> TPATQPLINAE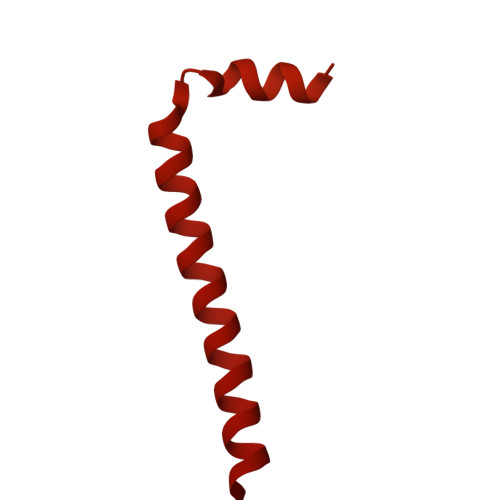PAVAAQTEQNPQVGQVMPGVQGADAPVVAQNGPSRDVKLTFAQIAPPPGSMVLRGINPNGSIEFGMRSDEVVTKAMLNLEYTPSPSLLPVQSQLKVYLNDELMGVLPVTKEQLGKKTLAQMPINPLFITDFNRVRLEFVGHYQDVCENPASTTLWLDVGRSSGLDLTYQTLNVKNDLSHFPVPFFDPRDNRTNTLPMVFAGAPDVGLQQASAIVASWFGSRSGWRGQNFPVLYNQLPDRNAIVFATNDKRPDFLRDHPAVKAPVIEMINHPQNPYVKLLVVFGRDDKDLLQAAKGIAQGNILFRGESVVVNEVKPLLPRKPYDAPNWVRTDRPVTFGELKTYEEQLQSSGLEPAAINVSLNLPPDLYLMRSTGIDMDINYRYTMPPVKDSSRMDISLNNQFLQSFNLSSKQEANRLLLRIPVLQGLLDGKTDVSIPALKLGATNQLRFDFEYMNPMPGGSVDNCITFQPVQNHVVIGDDSTIDFSKYYHFIPMPDLRAFANAGFPFSRMADLSQTITVMPKAPNEAQMETLLNTVGFIGAQTGFPAINLTVTDDGSTIQGKDADIMIIGGIPDKLKDDKQIDLLVQATESWVKTPMRQTPFPGIVPDESDRAAETRSTLTSSGAMAAVIGFQSPYNDQRSVIALLADSPRGYEMLNDAVNDSGKRATMFGSVAVIRESGINSLRVGDVYYVGHLPWFERLWYALANHPILLAVLAAISVILLAWVLWRLLRIISRRRLNPDNE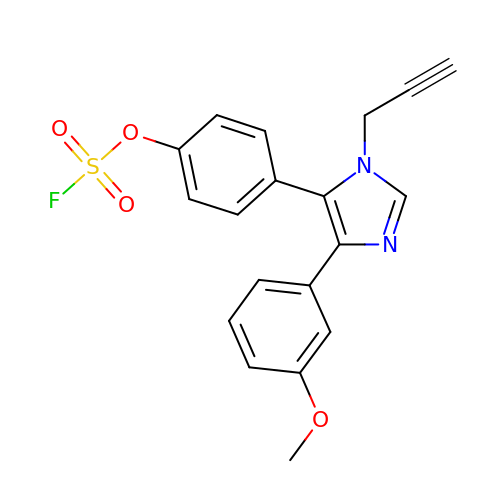4-[4-(3-methoxyphenyl)-1-(prop-2-yn-1-yl)-1H-imidazol-5-yl]phenyl sulfurofluoridate | C19 H15 F N2 O4 S | UQAHOPRAUGLTTO-UHFFFAOYSA-N> G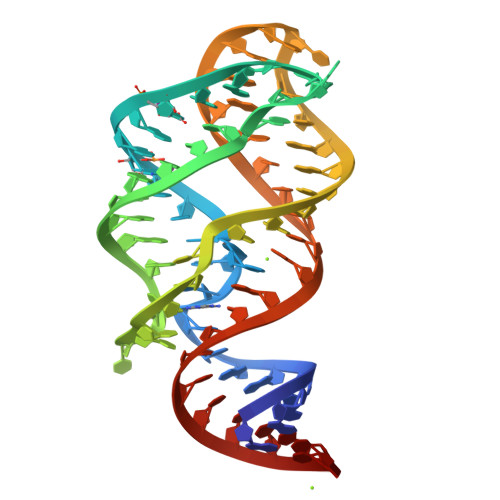GGAAGAUAUAAUCCUAAUGAUAUGGUUUGGGAGUUUCUACCAAGAGCCUUAAACUCUUGAUUAUCUUCCC> MFDYETLRFIWWLLIGVILVVFMISDGFDMGIGCLLPLVARNDDERRIVINSVGAHWEGNQVWLILAGGALFAAWPRVYAAAFSGFYVAMILVLCSLFFRPLAFDYRGKIADARW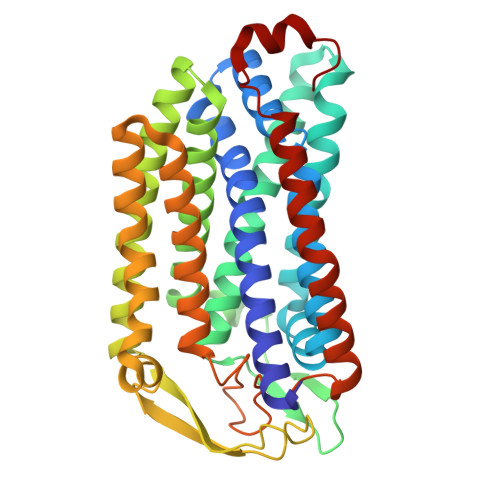RKMWDAGLVIGSLVPPVVFGIAFGNLLLGVPFAFTPQLRVEYLGSFWQLLTPFPLLCGLLSLGMVILQGGVWLQLKTVGVIHLRSQLATKRAALLVMLCFLLAGYWLWVGIDGFVLLAQDANGPSNPLMKLVAVLPGAWMNNFVESPVLWIFPLLGFFCPLLTVMAIYRGRPGWGFLMASLMQFGVIFTAGITLFPFVMPSSVSPISSLTLWDSTSSQLTLSIMLVIVLIFLPIVLLYTLWSYYKMWGRMTTETLRRNENELY> GP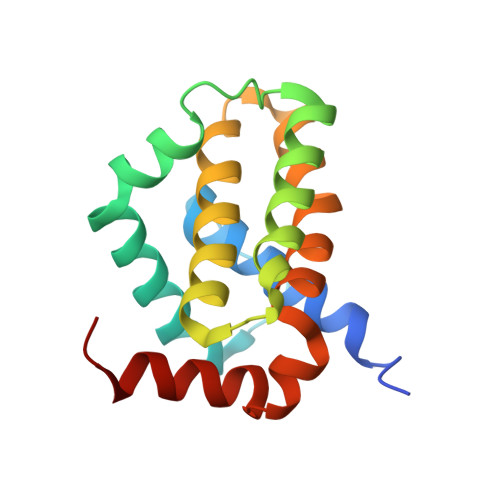LGSMDEDVLPGEVLAIEGIFMACGLNEPEYLYHPLLSPIKLYITGLMRDKESLFEAMLANVRFHSTTGINQLGLSMLQVSGDGNMNWGRALAILTFGSFVAQKLSNEPHLRDFALAVLPAYAYEAIGPQWFRARGGWRGLKAYCTQVLT>HHHHHHMKILFLDQSGKPGGAELCLIDIAKPYRDRALVGLFADGAFKTLLEQHHIPVEVFTNQPIQVRKQSNLLQAFGSLGQLAPLVAKVVQTAHEYDLIYANTQKALVVGAIASFIARRPLVYHLHDILSPEHFSQTNLRVAVNLANRFASLVIANSQASQTAFIQAGGRAELTKVIYNGFDINLYKTSPSDISKLRQQLGVANNFVVGHFSRLSPWKGQHILIDALAQCPPQVTAILVGDALFGEQDYVKELHQQIT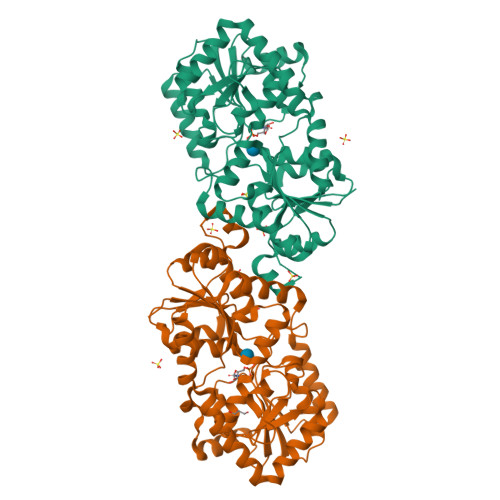RLGLENRVKFLGFRADIPQLMAACDLVAHTSTAPEPFGRVIVEAMLCGKPVVAAKAGGAMELVEHGVNGFLTTPGESQELANIINTCIEDTQKTATIASNAQAIASQRFDVVTINQQIAETLSSLGFTR[2x]> ATYHLEDNWVGSAFLSTFTHEAIADPTHGRVNYVDQATALAKNLTYASGDTLILRADHTTTLSPSGPGRNSVRIRSIKTYTTHVAVFDVRHMPQGCGTWPAAWETDEGDWPNGGEVDIIEGVNDQSPNAMTLHTGANCAMPASRTMTGHATNNNCDVNTDGNTGCGVQAPTANSYGPSFNANGGGWYAMERTNSFIKVWFFPRNAGNVPNDIASGPATINTDNWGTPTAFFPNTNCDI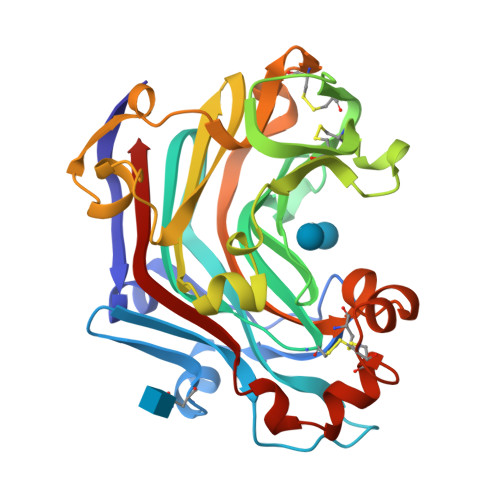GSHFDANNIIINLTFCGDWAGQASIFNGAGCPGSCVDYVNNNPSAFANAYWDIASVRVYQ> NTSLEAIVQNASSDNQGIQLSAVQAARKLLSSDRNPPIDDLIKSGILPILVHCLERDDNPSLQFEAAWALTNIASGTSEQTQAVVQSNAVPLFLRLLHSPHQNVCEQAVWALGNIIGDGPQCRDY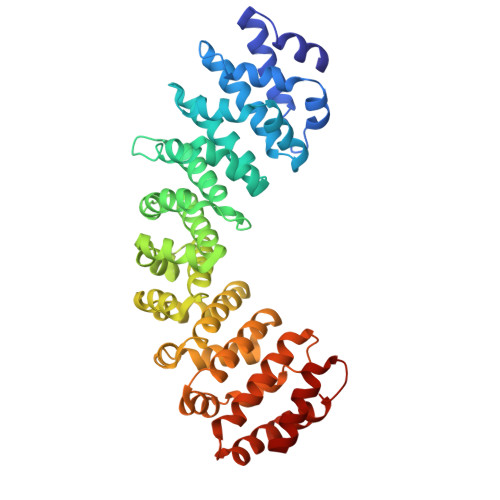VISLGVVKPLLSFISPSIPITFLRNVTWVMVNLCRHKDPPPPMETIQEILPALCVLIHHTDVNILVDTVWALSYLTDAGNEQIQMVIDSGIVPHLVPLLSHQEVKVQTAALRAVGNIVTGTDEQTQVVLNCDALSHFPALLTHPKEKINKEAVWFLSNITAGNQQQVQAVIDANLVPMIIHLLDKGDFGTQKEAAWAISNLTISGRKDQVAYLIQQNVIPPFCNLLTVKDAQVVQVVLDGLSNILKMAEDEAETIGNLIEECGGLEKIEQLQNHENEDIYKLAYEIIDQFF> MPSRAEDYEVLYTIGTGSYGRCQKIRRKSDGKILVWKELDYGSMTEAEKQMLVSEVNLLRELKHPNIVRYYDRIIDRTNTTLYIVMEYCEGGDLASVITKGTKERQYLDEEFVLRVMT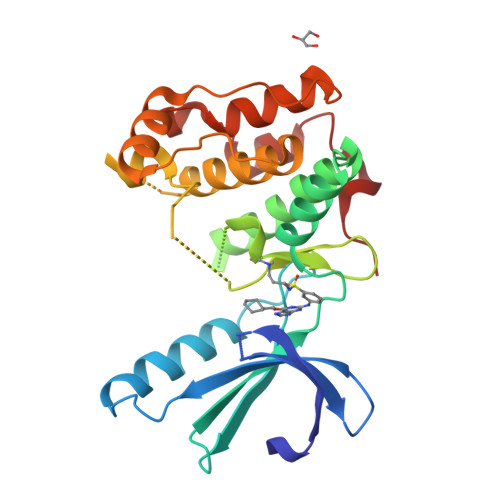QLTLALKECHRRSDGGHTVLHRDLKPANVFLDGKQNVKLGDFGLARILNHDTSFAKTFVGTPYYMSPEQMNRMSYNEKSDIWSLGCLLYELCALMPPFTAFSQKELAGKIREGKFRRIPYRYSDELNEIITRMLNLKDYHRPSVEEILENPLILEHHHHHH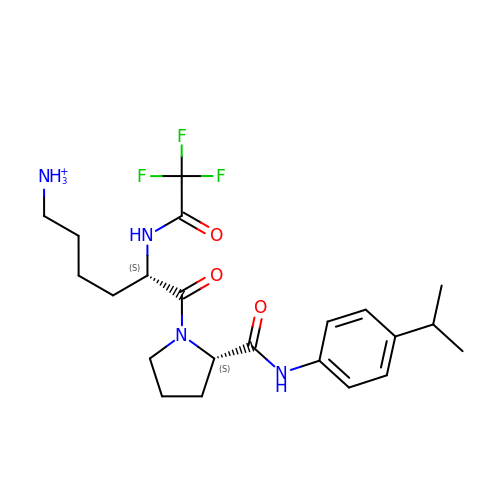6-ammonio-N-(trifluoroacetyl)-L-norleucyl-N-[4-(1-methylethyl)phenyl]-L-prolinamide | C22 H32 F3 N4 O3 | BEGRGCCTDSKILY-ROUUACIJSA-O> GAMGKVTHSIHIEKSDTAADTYGFSLSS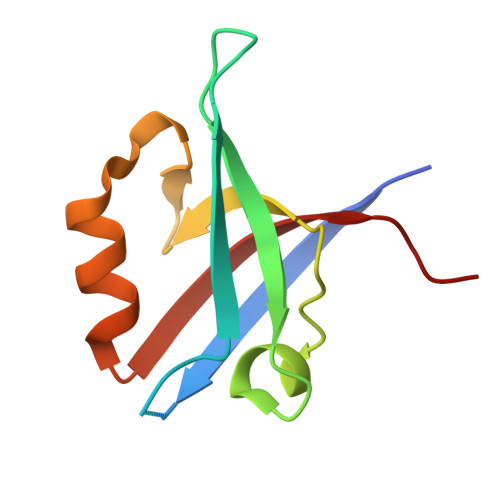VEEDGIRRLYVNSVKETGLASKKGLKAGDEILEINNRAADALNSSMMEDFFSQPSVGLLVRTYPEL> GSHMASEKKFSTEEEYVSPRFLVADGFLIDLAEEKPINPKDPRLLTLLKDHQRAMIDQMNLVKWNDFKKYQDPIPLKAKTLFKFCKQIKKKFLRGADFKLHTLPTEANLKYEPERMTVLASCVPILLDDQ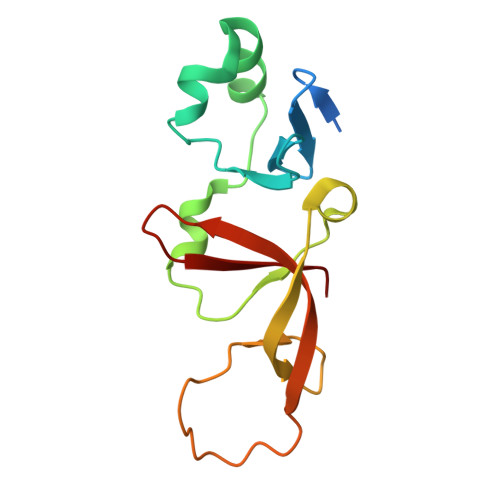TVQYLYDD>GSGIFPKVATNIMRAWLFQHLTHPYPSEEQKKQLAQDTGLTILQVNNWFINARRRIVQPMIDQSNR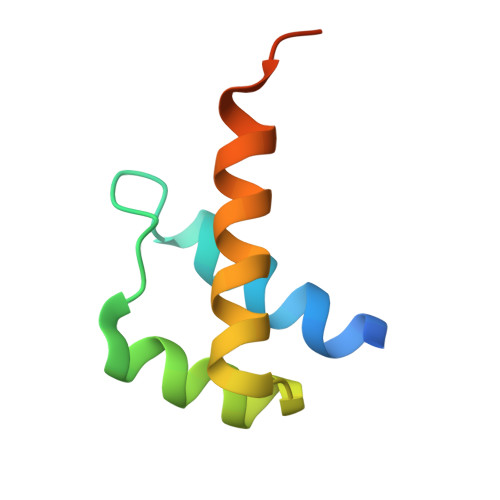A[8x]> MKYLLPTAAAGLLLLAAQPAMAMDSSGLEVLFQGPGSPGMAAPPVRLLPTNLAPHAVGELYRGPDQLVIGQREEDLAPVILDLAANPLLMVFGDARSGKTTLLRHIIRTVREHSTADRVAFTVLDRRLHLVDEPLFPDNEYTANIDRIIPAMLGLANLIEARRPPAGMSAAELSRWTFAGHTHYLIIDDVDQVPDSPAMTGPYIGQRPWTPLIGL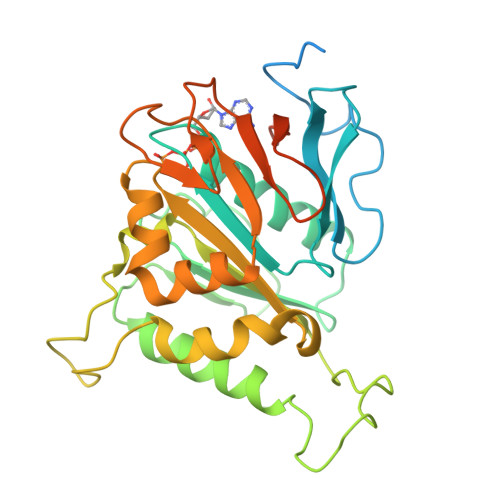LAQAGDLGLRVIVTGRATGSAHLLMTSPLLRRFNDLQATTLMLAGNPADSGKIRGERFARLPAGRAILLTDSDSPTYVQLINPLVDAAAVSGETQQKGSQSLEHHHHHH>[4x]SNAASLVHQPHPLEHSWTFWFDNPSAKSKQATWGASIRPIYTFSTVEEFWSVYNNIHHPSKLAMRADLYCFKHKIEPKWEDPVCAN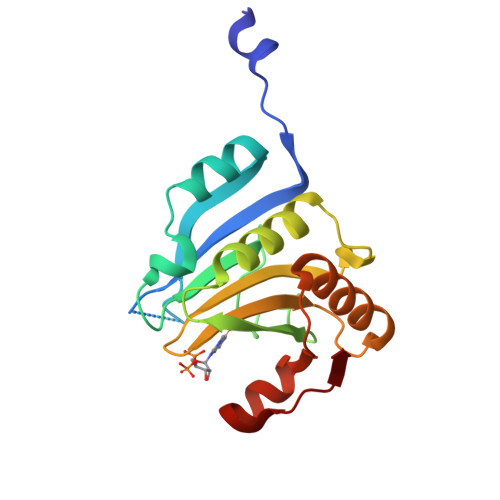GGKWTVNFPRGKSDNGWLYTLLAMIGEQFDCGDEICGAVVNVRSGQDKISIWTKNASNEAAQASIGKQWKEFLDYNESIGFIFHDDAKKFDRHAKNKYMV(R)-4-hydroxy-2-pyrrolidone | C4 H7 N O2 | 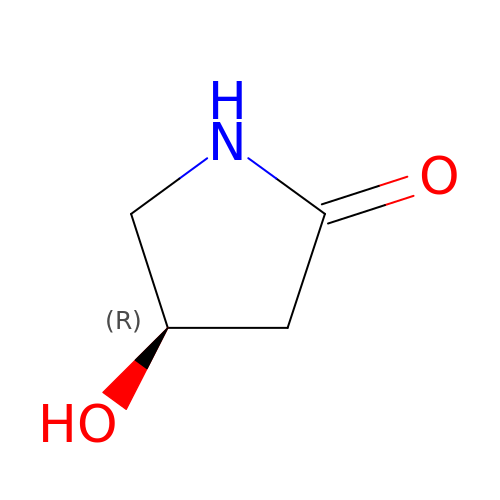IOGISYQVOGVIEU-GSVOUGTGSA-N>MQANGAGGGGGGGGGGGGGGGGGGGQGQTPELACLSAQNGESSPSSSSSAGDLAHANGLLPSAPSAASNNSNSLNVNNGVPGGAAAASSATVAAASATTAASSSLATPELGSSLKKKKRLSQSDEDVIRLIGQHLNGLGLNQTVDLLMQESGCRLEHPSATKFRNHVMEGDWDKAENDLNELKPLVHSPHAIVRMKFLLLQQKYLEYLEDGKVLEALQVLRCELTPLKYNTERIHVLSGYLMCSHAEDLRAKAEWEGKGTASRSKLLDKLQTYLPPSVMLPPRRLQTLLRQAVELQRDRCLYHNTKLDNNLDSVSLLIDHVCSRRQFPCYTQQILTEHCNEVWFCKFSNDGTKLATGSKDTTVIIWQVDPDTHLLKLLKTLEGHAYGVSYIAWSPDDNYLVACGPDDCSELWLWNVQTGELRTKMSQSHEDSLTSVAWNPDGKRFVTGGQRGQFYQCDLDGNLLDSWEGVRVQCLWCLSDGKTVLASDTHQRIRGYNFEDLTDRNIVQEDHPIMSFTISKNGRLALLNVATQGVHLWDLQDRVLVRKYQGVTQGFYTIHSCFGGHNEDFIASGSEDHKVYIWHKRSELPIAELTGHTRTVNCVSWNPQIPSMMASASDDGTVRIWGPAPFIDHQNIEEECSSMDS[2x];> MGRIFLDHIGGTRLFSCANCDTILTNRSELISTRFTGATGRAFLFNKVVNLQYSEVQDRVMLTGRHMVRDVSCKNCNSKLGWIYEFATEDSQRYKEGRVILERALVRESEGFEEHVPSDNS

Here, we discover that human WDR26 binds the metabolic enzyme NMNAT1 and mediates its CTLH E3-dependent ubiquitylation independently of canonical GID/CTLH E3-family substrate receptors. Cryo-EM structures of NMNAT1- and YPEL5-bound WDR26-CTLH E3 assemblies reveal an internal basic degron motif of NMNAT1 essential for targeting by WDR26-CTLH E3, and degron mimicry by YPEL5’s N-terminus antagonizing substrate targeting. Cryo-EM structures reveal that WDR26 acts as a non-interchangeable substrate receptor for NMNAT1. Within the supramolecular WDR26-CTLH E3 assembly, the WD40-repeat β-propeller domains from two WDR26 dimers are exposed and provide multiple binding surfaces for NMNAT1.

Cryo-EM maps revealed how YPEL5 inhibits substrate targeting: there is structural overlap between YPEL5 and NMNAT1 binding sites on WDR26-CTLH. Molecular details of YPEL5 binding to WDR26 were revealed by a 3.2-Å-resolution focused refined map. Our structural analysis revealed multivalent binding of a single YPEL5 to both WDR26 β-propeller domains in a WDR26 dimer. YPEL5’s N-terminus presents a sequence that mimics NMNAT1’s internal basic motif that together with YPEL5’s C-terminus captures one WDR26 protomer. Meanwhile, YPEL5’s globular domain binds the adjacent WDR26 protomer. As such, YPEL5 modulates WDR26’s accessibility to degrons from bona fide substrates. From YPEL5, the N-amino group of G2 (exposed upon cleavage of initiator M1) and the side chains of R3 and F5 are anchored through a similar constellation of electrostatic and hydrophobic contacts as the γ-amino group of K126 side chain, R127 and W129 from NMNAT1basic. Comparing the NMNAT1basic and YPEL5 N-terminal sequences reveals a consensus G/K-R-X-ϕ basic motif (ϕ represents amino acids with a bulky hydrophobic residue including W, Y, F) that might be selectively recognized by WDR26. Whereas YPEL5-HA efficiently co-precipitate WDR26, binding to WDR26 was completely abolished in the absence of YPEL5’s N-terminus. Taken together, we propose that YPEL5 inhibits WDR26’s substrate receptor function by mimicking internal basic substrate degrons, thereby preventing substrate ubiquitin targeting.> PLSFQNPLF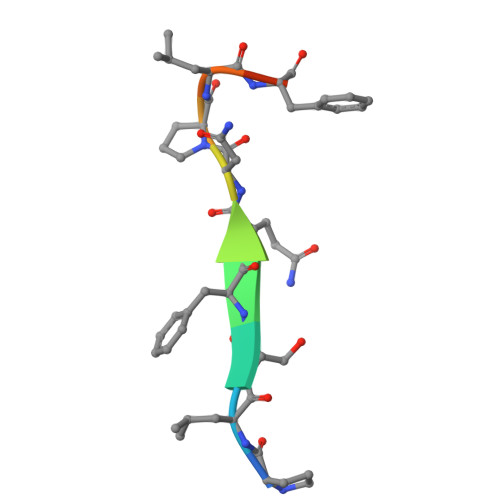HM>[2x]KPGDIFEVELAKNDNSLGISVTGGVNTSVRHGGIYVKAVIPQGAAESDGRI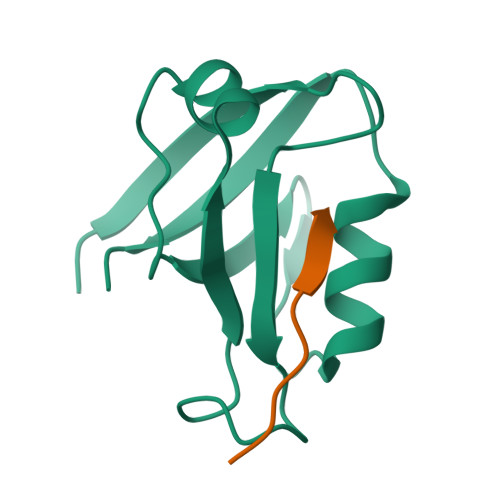HKGDRVLAVNGVSLEGATHKQAVETLRNTGQVVHLLLEKGQSPT;>RHSGSYLVTSV[2x]>[2x]AGSAVPFHGAHQAGIATPVQDRLHFAAFDVTTEDRAAFVALLKEWTAAARRLTAGHAVGEGAYGGLPEAPPDDTGEALGLKPSRLTLTIGFGPSLFTRFGLADLRPEALADLPKFPGDNLDRARSGGDLCVQA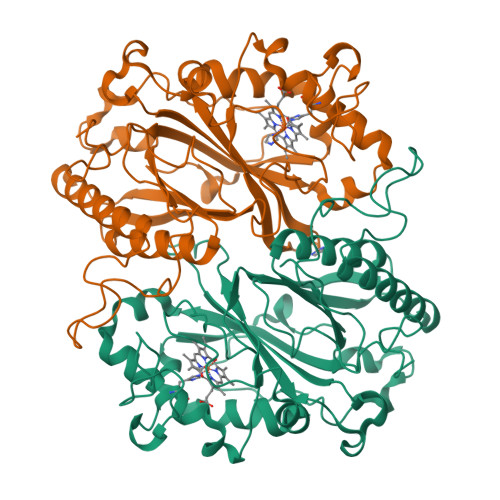CADDPQVAVHAIRNLARIGFGKVVVRWSQLGFGKTSSTTPDKQTPRNLLGFKDGTRNIAGTEKDRLDRFVWAAEKDGTPWMTGGSYLVARRIRMHIETWDRASLQEQEDVFGRDKGEGAPVGKAKERDEPFLKAMKPDAHVRLAHPDSNGGATLLRRGYSFTDGTDGLGRLDAGLFFLAYQRDIRTGFVPVQRNLATDALNEYIQHVGSAVFAVPPGVRDADDWWGSTLF>[18x]MSVLTIGDKRLGAALLDAGLLTDEELQRALERHREVGGSLAEVLVDMGLLSERRIAQTIEDRFGIPLVELHRVEIPPKVKALLPAEKAKELKAIPFALDEEAGVVRVAFLNPLDTLSLEEVEDLTGLVVEPYQTTKSAFLYALAKHYPELGLPVPPPPSGEGQKDLKLGELLLQKGWISREALEEALVEQEKTGDLLGRILVRKGLPEEALYRALAEQKGLEFLESTEGIVPDPSAALLLLRSDALRYGAVPIGFQNGEVEVVLSDPRHKEAVAQLLNRPARFYLALPQAWEELFRRAYPQKNRLGEVLVQEGKLSREALKEALEVQKGLPRAKPLGEILVELGLARPEDVEEALQKQRRGGGRLEDTLVQSGKLRPEALAQAVATQLGYPYVDPEEDPPDPGAPLLLPEDLCRRYGVFPHRLEGNRLVLLMKDPRNILALDDVRLALKRKGLNYEVAPAVATEAAITKLIERFYGKAELSEIAKEFAKKQAEEEVPSPLELDESAAQKFVKQVIREAFLQDASDIHIEPRQNDVQVRLRIDGALRPYSTLPKGALNAVISVVKIMGGLNIAEKRLPQDGRVRYREGAIDVDLRLSTLPTVYGEKAVMRLLKKASDIPEIEDLGFAPGVFERFKEVISKPYGIFLITGPTGSGKSFTTFSILKRIATPDKNTQTIEDPVEYEIPGINQTQVNPQAGLTFARALRAFLRQDPDIIMVGEIRDSETAKIATEAALTGHLVIATLHTNDAAQAITRLDEMGVEPFNISAALIGVLSQRLVRRVCEHCKVEVKPDPETLRRLGLSEAEIQGARLYKGMGCERCGGTGYKGRYAIHELLVVDDEIRHAIVAGKSATEIKEIARRKGMKTLREDGLYKALQGITTLEEVLARTIEAAAELALVPRGSSAHHHHHHHHHH

A third vital component of the TFP biogenesis system is the assembly ATPase (PilF in T. thermophilus). The TFP assembly ATPases are part of the extensive AAA+ superfamily which form molecular motors, using the energy from ATP hydrolysis to drive mechanical transformations. The domain structure of T2SS and TFP biogenesis ATPases is similar, in that they comprise one or more N1 or GSPII domains at the N-terminus, followed by a C-terminal (CTD) and N2 domain- which comprise the ATP binding site. Here we present a combination of X-ray crystallographic and cryoelectron microscopy single particle reconstructions of the PilF hexamer in two states which are used to build molecular models for the complete PilF hexamer and chart its structural transition on binding of ATP.

Estimation of the resolution of the TtPilF map (AMPPNP-bound form) by FSC correlation gave a value of 8 Å at the conservative value of 0.5. To construct a molecular model for the TtPilF hexamer, we examined the fitting of the TtPilFc crystal structure into the AMPPNP cryoelectron density map. The correctly docked form was readily identified by a superior correlation coefficient (0.83 versus 0.70), which reflected a much better fit of the crystal structure into the top half of the density map. The fit of the docked model was optimized by refinement in ROSETTA27, giving the model TtPilFAMPPNP. The results were indicative of 12 separate domains in the lower half of the PilF hexamer i.e. two domains per TtPilF chain. The model of the TtPilF cylinder is formed from two rings, each containing 6 N1 domains; the N1 domains are orientated such that the four α-helix subdomains lie on the outside of the cylinder. Calculations of centers of mass for each domain showed that the TtPilFAMPPNP N1 domains from both ring 1 and ring 2 are displaced downwards by distances of 4–9 Å. This is accompanied by rotation outwards (mean value 14o for ring 2 domains), which leads to a wider aperture at the base of the structure. Binding of AMPPNP is accompanied by an outward expansion of the CTD and N2 domains which is linked to a downward and outwards displacement of N1 domains on binding of AMPPNP.>[2x]GSHMKNSVSVDLPGSMKVLVSKSSNADGKYDLIATVDALELSGTSDKNNGSGVLEGVKADASKVKLTISDDLGQTTLEVFKSDGSTLVSKKVTSGGS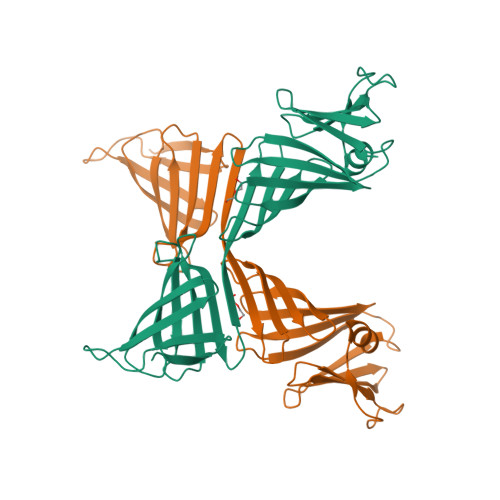STEEKTTTEKIITRADGTRLEYTGIKSDGSGKAKEVLKGYVLEGTLTAEKTTLVVKEGTVTLSKNISKSGEVSVELNDTDSSAATKKTAAWNSGTSTLTITVNSKKTKDLVFTSSNTITVQQYDSNGTSLEGSAVEITKLDEIKNALK>[2x]GHHHHHH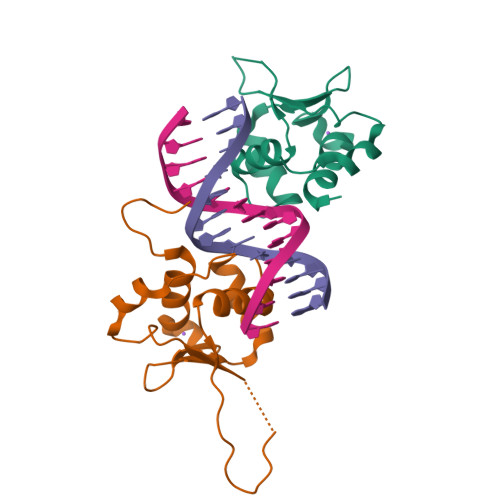VPAFLTKLWTLVSDPDTDALICWSPSGNSFHVFDQGQFAKEVLPKYFKHNNMASFVRQLNMYGFRKVVHIEQGGLVKPERDDTEFQHPCFLRGQEQLLENIKRKVT>ASNLKIVRMDRTAGCVTGGEEIYLLCDKVQKDDIQIRFYEEEENGGVWEGFGDFSPTDVHRQFGIVFKTPKYKDVNITKPASVFVQL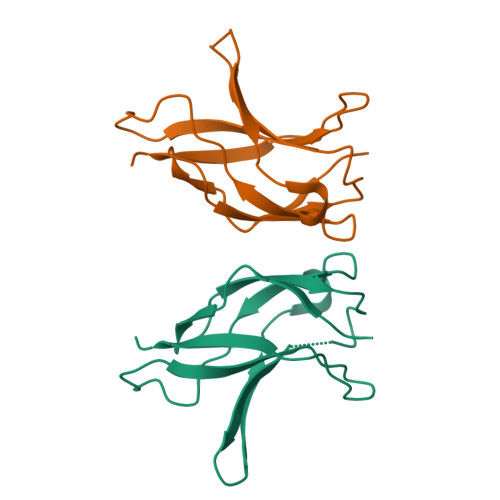RRKSDLETSEPKPFLYYPE[4x]>[2x]GGFDYDVVVVGGGFAGATAARECGLQGYRTLLLEARSRLGGRTFTSRFAGQEIEFGGAWVHWLQPHVWAEMQRYGLGVVEDPLTNLDKTLIMYNDGSVESISPDEFGKNIRIAFEKLCHDAWEVFPRPHEPMFTERARELDKSSVLDRIKTLGLSRLQQAQINSYMALYAGETTDKFGLPGVLKLFACGGWNYDAFMDTETHYRIQGGTIGLINAMLTDSGAEVRMSVPVTAVEQVNGGVKIKTDDDEIITAGVVVMTVPLNTYKHIGFTPALSKGKQRFIKEGQLSKGAKLYVHVKQNLGRVFAFADEQQPLNWVQTHDYSDELGTILSITIARKETIDVNDRDAVTREVQKMFPGVEVLGTAAYDWTADPFSLGAWAAYGVGQLSRLKDLQAAEGRILFAGAETSNGWHANIDGAVESGLRAGREVKQLLSLEH

The nicotine oxidoreductase NicA2 is a crucial enzyme for the first step of nicotine degradation in Pseudomonas putida S16 (DSM 28022). NicA2 from P. putida S16, 6HLNO and 6HDNO from A. nicotinovorans, and the nicotine oxidase NOX from Pseudomonas sp. strain HZN6 (21) belong to the family of flavin-dependent amine oxidases. In the NicA1- or NicA2-catalyzed reaction, flavin adenine dinucleotide (FAD) is required as a cofactor to couple the oxidation of nicotine with the reduction of oxygen to hydrogen peroxide. The structure of NicA2 comprises a FAD-binding domain (residues 49 to 129, 250 to 338, and 417 to 482) that harbors the cofactor FAD and a substrate-binding domain (residues 130 to 249 and 339 to 416) associated with the substrate nicotine.

To understand the molecular recognition mechanism of NicA2 for its cofactor FAD and the substrate nicotine, we first determined the crystal structure of selenomethionine (SeMet)-substituted NicA2 residues 21 to 482 [NicA2(21–482)] in complex with FAD at 2.05 Å resolution using the single-wavelength anomalous dispersion (SAD) method. An N-terminal cut and SeMet substitution were performed to improve the quality and resolution of the crystals. In both structures, there are two complexes in each asymmetric unit. However, as demonstrated by gel filtration chromatography, NicA2 behaves as a monomer in solution. The FAD cofactor adopts an extended conformation deeply inserted into the FAD-binding domain. FAD is tightly associated with NicA2 through extensive interactions between FAD and the FAD-binding domain. NicA2 presents as yellow in solution, which is consistent with the presence of FAD as the cofactor.>[3x]GPTDFENTGKIQLNPVLVSTDIGKKNVAKNLGEGNMRLTGKLVRYGDNLTFSGVANAGKELVIDVTELGYYTLELTLADNENIIQTAVVNYAVVPEIIDEERPLDMGVCVHPPKDNDYSKTFRLIRMAGFTRIRTDLAWEHVEPAKGKYVMPEHMYQFVSASEKEGIKPLIVFGYANAIAYPNGFPTIPFPTTEESRLGCANALAYAVKEMGNRVTEWELWNEPNYADPVKDYLPLLKVVYPTVKKVNPDITLISGGGSGAGGGPGGAFIIPVLDAGGVDFQDGYSIHPYMAPNTPDFGYAGTGGPIPAVNIPTVWPYLKKISEENL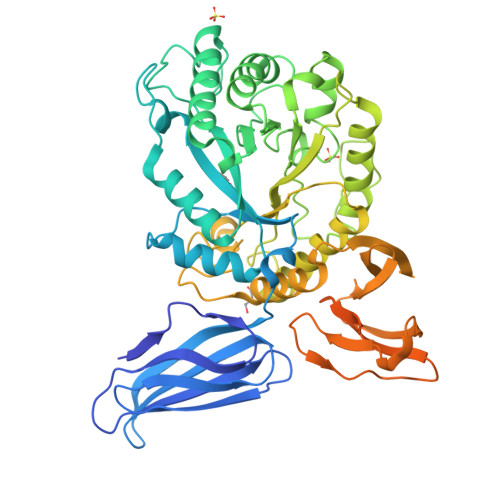RSDKKELSVWVTEIGWNSTTNLDIEQAAYLARTYLLSRRHYMSPGVFWYDFQNDGDTPDNIEHNFGLLRSDFSPKPSYQAAAVVASLLKNYTFQETLLDGVNKVLAFGQDGETTFYTAWTTKAEGTTIRVKAPTDVDKLRLIDWQGCEMPLTVDNGYLVLNLSILPQYLVVKEEVVGITSPVGKAGIKLYPNPSTGLLIVNWGHEGNRTITINDLNGRILQRKVTYGLETQMNISDLNAGIYMLCVNDGKEQVTLKVIKQ~{N}-[1,1-bis(oxidanylidene)thian-4-yl]-7-[3-methyl-1-(piperidin-4-ylmethyl)indol-5-yl]-4-oxidanylidene-5-propyl-thieno[3,2-c]pyridine-2-carboxamide | C31 H38 N4 O4 S2 | 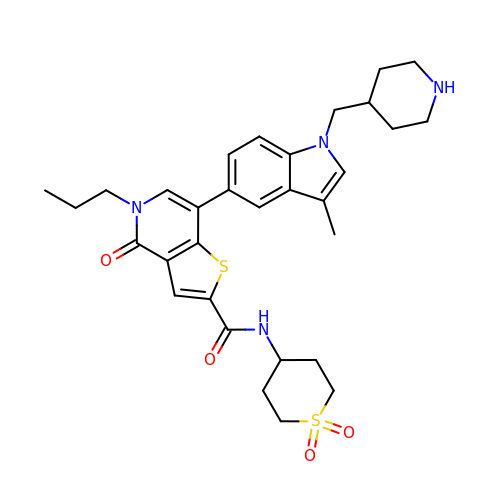VJSZEIHADFWXCN-UHFFFAOYSA-N>[2x]RSPWCVICDPSVVLALKSLEKDYLPGHLDAKHHKAMMERVENAVKDFQEL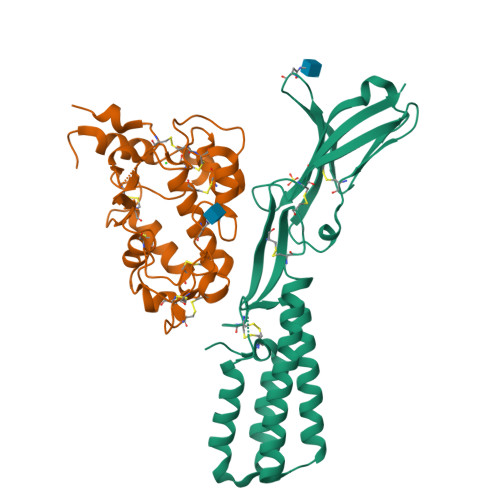SLNEDAYMGVVDEATLQKGSWSLLKDLKRITDSDVKGDLFVKELFWMLHLQKETFATYVARFQKEAYCPNKCGVMLQTLIWCKNCKKEVHACRKSYDCGERNVEVPQMEDMILDCELNWHQASEGLTDYSFYRVWGNNTETLVSKGKEATLTKPMVGPEDAGSYRCELGSVNSSPATIINFHVTVLPKEFLEVLFQ;>RSPWGDELLNICMNAKHHKRVPSPEDKLYEECIPWKDNACCTLTTSWEAHLDVSPLYNFSLFHCGLLMPGCRKHFIQAICFYECSPNLGPWIQPVGSLGWEVAPSGQGERVVNVPLCQEDCEEWWEDCRMSYTCKSNWRGGWDWSQGKNRCPKGAQCLPFSHYFPTPADLCEKTWSNSFKASPERRNSGRCLQKWFEPAQGNPNVAVARLFASEFLEVLFQ[2x]> SVDDEPIRLPNPMIGFGVPNEPGLITHRSLPELARGPPFFYYENVALTPKGVWETISRHLFEIPPEFVDSKYFCVAARKRGYIHNLPINNRFQIQPPPKYTIHDAFPLSKRWWPEWDKRTKLNCILTCTGSAQLTNRIRVALEPYNEEPEPPKHVQRYVIDQCKKWNLVWVGKNKAAPLEPDEMESILGFPKNHTRGGGMSRTERFKSLGNSFQVD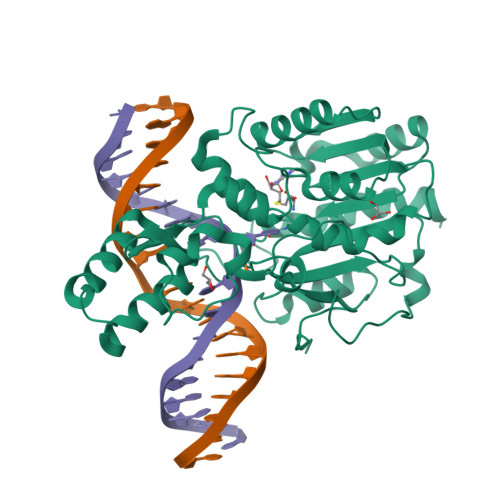TVAYHLSVLKPIFPHGINVLSLFTGIGGGEVALHRLQIKMKLVVSVEISKVNRNILKDFWEQTNQTGELIEFSDIQHLTNDTIEGLMEKYGGFDLVIGGSPCNNLAGGNRVSRVGLEGDQSSLFFEYCRILEVVRARMRGS> GEFLATTLERIEKNFVITDPRLPDNPIIFASDSFLQLTEYSREEILGRNCRFLQGPETDRATVRKIRDAIDNQTEVTVQLINYTKSGKKFWNLFHLQPMRDQKGDVQYFIGVQLDGTEHVRDAA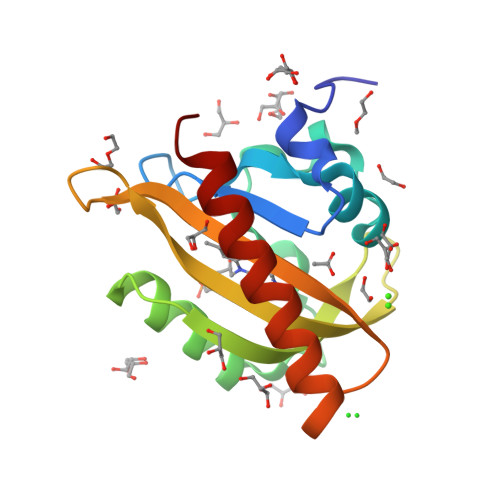EREGVMLIKKTAENIDEAAKEL> MSGSFWTSTQRHHWQYTKASLAKERQKLWLLECQLFPQGLNIVMDSKQNGIEQSITKNIPITHRDLHYDKDYNLRIYCYFLIMKLG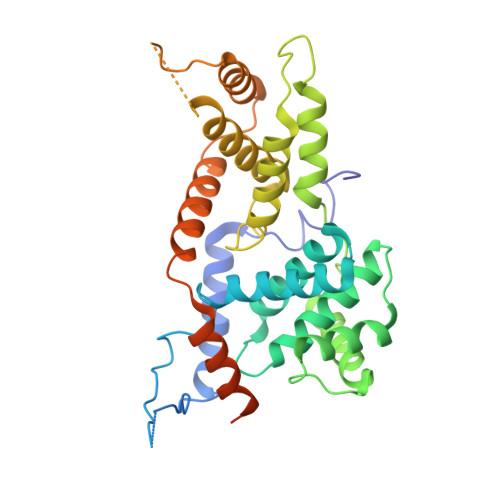RRLNIRQYALATAHIYLSRFLIKASVREINLYMLVTTCVYLACKVEECPQYIRTLVSEARTLWPEFIPPDPTKVTEFEFYLLEELESYLIVHHPYQSLKQIVQVLKQPPFQITLSSDDLQNCWSLINDSYINDVHLLYPPHIIAVACLFITISIHGKPTKGSSLASAASEAIRDPKNSSSPVQIAFNRFMAESLVDLEEVMDTIQEQITLYDHWDKYHEQWIKFLLHTLYLRPASAISMEKRRWKKNFIAVSAANRFKKISSSGAL> MSASQSSMSGAGEPGARAVVWFRRDLRVEDNPALAAAARAAGEVVPAYVWAPEEDGAYYPGRVSRWWLSQSLKHLDASLRRLGAARLVTRRSNDAVAALLDLVRCTGATHLFFNHLYDPLSLVRDYRVKEQLAAEGIDVQSFNADLLYEPWEVLDEDRRPFTMFAPFWNRCLCMPDPAAPLLPPKRINSGDLSRCPWDELVFEDESERGSNALLARAWSPGWQNADKALTAFLNGPLMDYSVNRKKADSASTSLLSPYLHFGELSVRKVFHQVRMKQLMWSNDGNHAGEESCTLFLRSIGLREYSRYLTFNHPCSHEKPLLSHLRFFPWVVN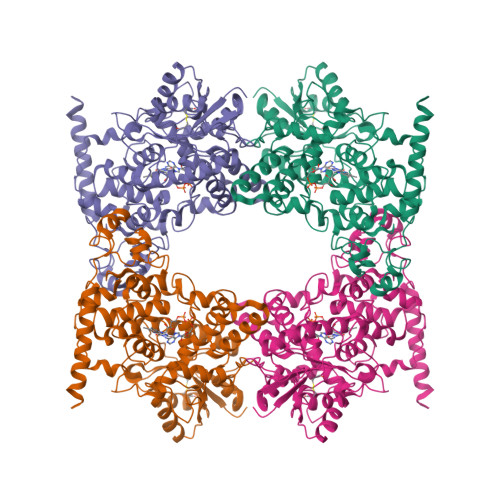EVYFKVWRQGRTGYPLVDAGMRELWATGWVHDRIRVVVSSFFVKVLQLPWRWGMKYFWDTLLDADLESDALGWQYISGSLPDGRELDRIDNPQFEGYKFDPHGEYVRRWLPELARLPTEWIHHPWDAPESVLQAAGVELGSNYPRPIVELDAANSRLQDALSEMWELEAASRA> NNNGACUUA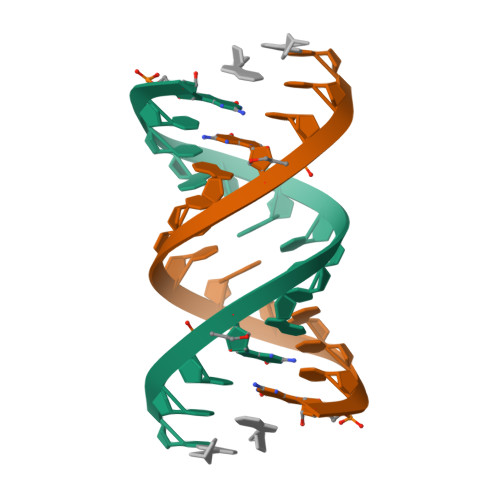AGUCG;>[2x]GG> GSHMKNSVSVDLPGSMKVLVSKSSNADGKYDLIATVDALELSGTSDKNNGSGVLEGVKADASKVKLTISDDLGQTTLEVFKSDGSTLVSKYVTSKDKSSTYEKFNEKGEVSEKYITRADGTRLEYTGIKSDGSGKAKEVLKGYVLEGTLTAEKTTLVVKEGTVTLSKNISKSGEVSVELNDTDSSAATKKTAAWNSGTSTLTITVNSKKTKDLVFTSSNTITVQQYDSNGTSLEGSAVEITKLDEIKNA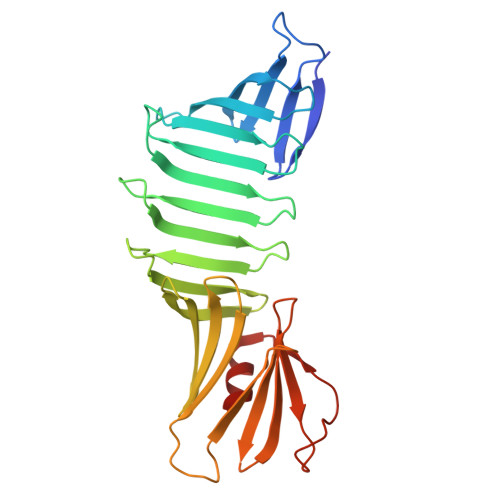LK>MYKCLIWGVNDEYTLAYDKLLFEISKGNLSIEALISKDKYAKYIDGKEVIDKTEISNYEFDYIIIFNKERYSDIK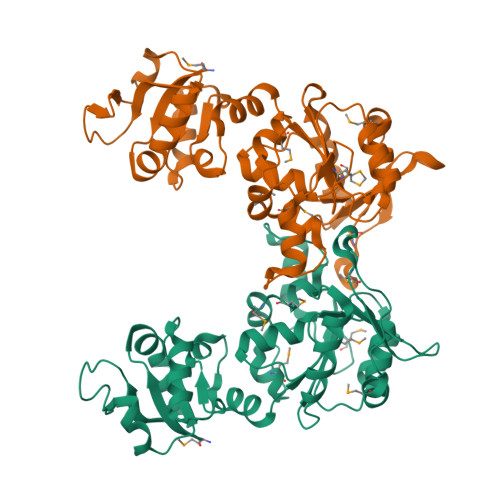NEALELGIPERKILNGKFFFISNFDFKRYCKLIENPITIISDDCWGGLVSSYLGFKFNSPFINFYIHNDDYIKFLENMDYYLEQELKVEQEGNVYSCTMPKGSLGTGDNKIILNFNHQASFAEAKNDWDERKTRINKKNLFVKMLIKDDNEKLVKRFDNLPYKNKVCFHPKPMKYKSVAFFPRYIWRCINYAARTSNSNLEQYTMDMSWLEKSCDILKMLCGEEDFIREKX[2x]4-[4-[2,4-bis(fluoranyl)phenyl]piperazin-1-yl]-2-fluoranyl-N-[(2R)-3-(1H-indol-3-yl)-1-oxidanylidene-1-(pyridin-4-ylamino)propan-2-yl]benzamide 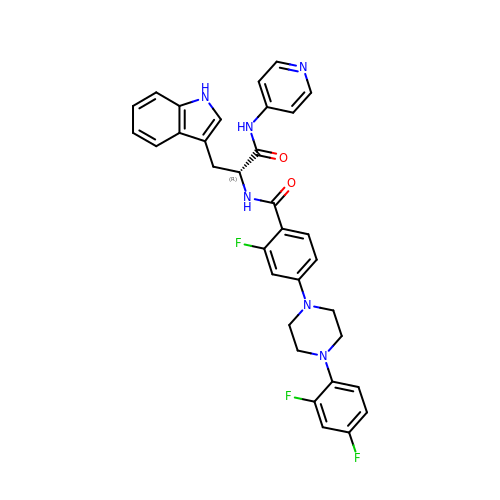| C33 H29 F3 N6 O2 | WRESLWUWFGDSMV-SSEXGKCCSA-N> GLPVMTTPGSTQFLTSDDFQSPSAMPQFDVTPEMQIPGRVNNLMEIAEVDSVVPVNNTEANVNSLKAYQIPVQSNSDNGKQVFGFPLQPGANGVLNRTLLGEILNYYTHWSGSIKLTFMFCGSAMATGKFLLAYSPPGAGVPKNRKDAMLGTHVIWDVGLQSSCVLCVPWISQT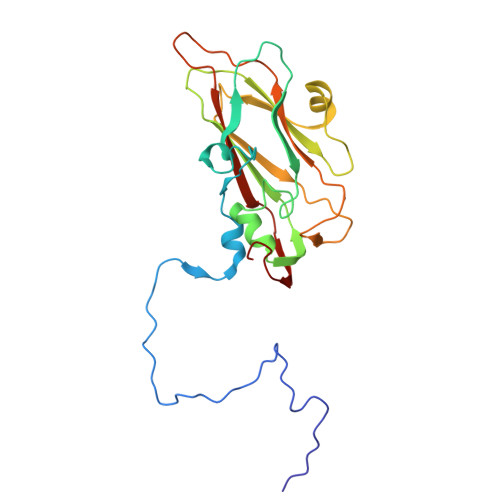HYRYVVEDEYTAAGYITCWYQTNIVVPADVQSSCDILCFVSACNDFSVRMLKDTPFIR>[2x]ALYEDPPDQKTSPSGKPATLKICSWNVDGLRAWIKKKGLDWVKEEAPDILCLQQTKCSENKLPAELQELPGLSHQYWSAPSDKEGYSGVGLLSRQAPLKVSYGIGDEEHDQEGRVIVAEFDSFVLVTAYVPNAGRGLVRLEYRQRWDEAFRK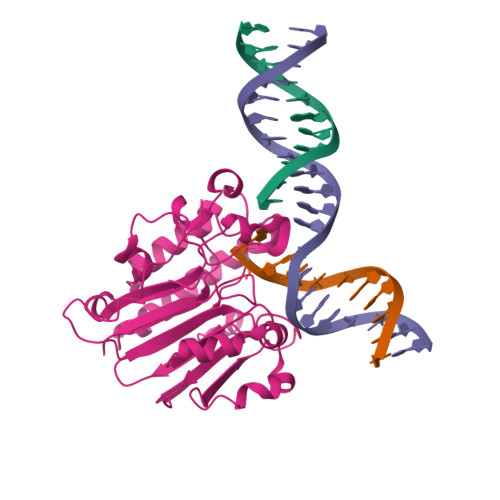FLKGLASRKPLVLCGNLNVAHEEIDLRNPKGNKKNAGFTPQERQGFGELLQAVPLADSFRHLYPNTPYAYTFWTYMMNARSKNVGWRLDYFLLSHSLLPALCDSKIRSKALGSDHCPITLYLAL>GSHMSKAFDLVVIGAGSGGLEAGWNAATLYGKRVAVVDVQTSHGPPFYAALGGTCVNVGCVPKKLMVTGAQYMDHLRESAGFGWEFDGSSVKANWKKLIAAKNEAVLDINKSYEGMFNDTEGLDFFLGWGSLESKNVVVVRETADPKSAVKERLQADHILLATGSWPQMPAIPGIEHCISSNEAFYLPEPPRRVLTVGGGFISVEFAGIFNAYKPPGGKVTLCYRNNLILRGFDETIREEVTKQLTANGIEIMTNENPAKVSLNTDGSKHVTFESGKTLDVDVVMMAIGRIPRTNDLQLGNVGVKLTPKGGVQVDEFSRTNVPNI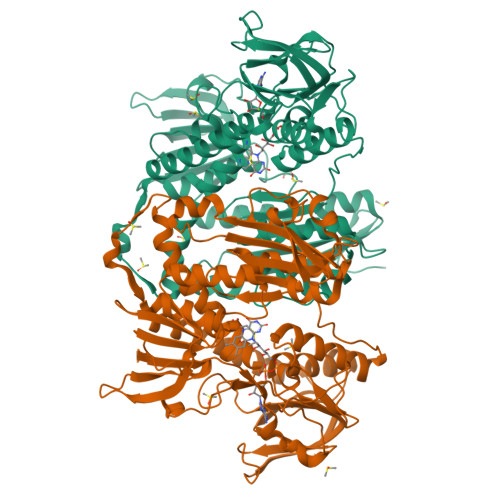YAIGDITDRLMLTPVAINEGAALVDTVFGNKPRKTDHTRVASAVFSIPPIGTCGLIEEVAAKEFEKVAVYMSSFTPLMHNISGSKYKKFVAKIVTNHSDGTVLGVHLLGDGAPEIIQAVGVCLRLNAKISDFYNTIGVHPTSAEELCSMRTPSYYYVKGEKMEKLPDSNL[2x]>[4x]KPYNKIVSHLLVAEPEKIYAMPDPTVPDSDIKALTTLCDLADRELVVIIGWAKHIPGFSTLSLADQMSLLQSAWMEILILGVVYRSLSFEDELVYADDYIMDEDQSKLAGLLDLNNAILQLV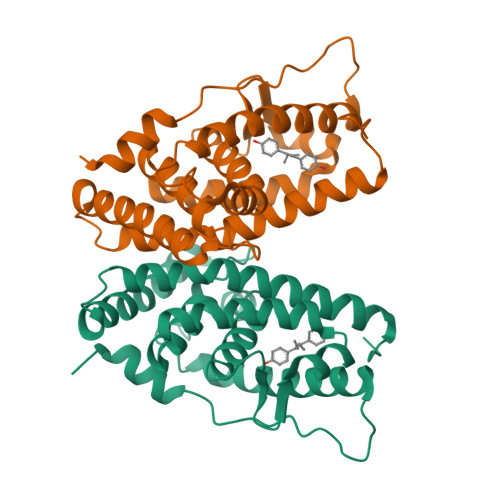KKYKSMKLEKEEFVTLKAIALANSDSMHIEDVEAVQKLQDVLHEALQDYEAGQHMEDPRRAGKMLMTLPLLRQTSTKAVQHFYNIKLEGKVPMHKLFLEMLEAKV> HHHHHHHMTAPAADDRI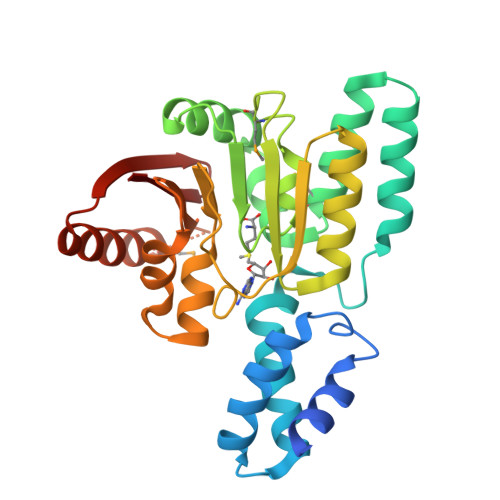DEIERAITKSRRYQTVAPATVRRLARAALVAARGDVPDAVKRTKRGLHEIYGAFLPPSPPNYAALLRHLDSAVDAGDDEAVRAALLRAMSVHISTRERLPHLDEFYRELFRHLPRPNTLRDLACGLNPLAAPWMGLPAETVYIASDIDARLVGFVDEALTRLNVPHRTNVADLLEDRLDEPADVTLLLKTLPCLETQQRGSGWEVIDIVNSPNIVVTFPTKSLGQRSKGMFQNYSQSFESQARERSCRIQRLEIGNELIYVIQK> RPPNIVLIFADDLGYGDLGCYGHPSSTTPNLDQLAAGGLRFTDFYVPVSLGTPSRAALLTGRLPVRMGMYPGVLVPSSRGGLPLEEVTVAEVLAARGYLTGMAGKWHLGVGPEGAFLPPHQGFHRFLGIPYSHDQGPCQNLTCFPPATPCDGGCDQGLVPIPLLANLSVEAQPPWLPGLEARYMAFAHDLMADAQRQDRPFFLYYASHHTHYPQFSGQSFAERSGRGPFGDSLMELDAAVGTLMTAIGDLGLLEETLVIFTADNGPETMRMSRGGCSGLLRCGKGTTYEGGVREPALAFWPGHIAPGVTHELASSLDLLPTLAALAGAPLPNVTLDGFDLSPLLL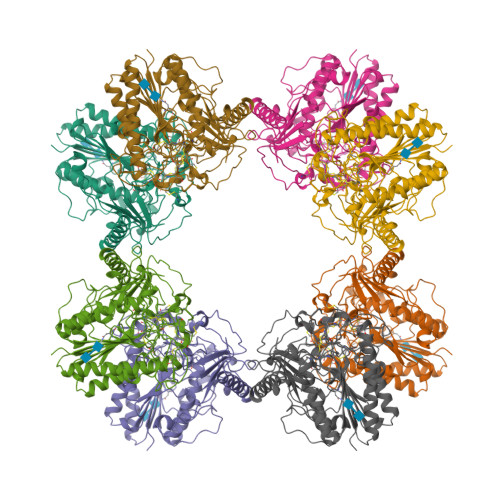GTGKSPRQSLFFYPSYPDEVRGVFAVRTGKYKAHFFTQGSAHSDTTADPACHASSSLTAHEPPLLYDLSKDPGENYNLLGGVAGATPEVLQALKQLQLLKAQLDAAVTFGPSQVARGEDPALQICCHPGCTPRPACCHCPDPHA>GQDMVSPPPPIADEPLTVNTGIYLIECYSLDDKAETFKVNAFLSLSWKDRRLAFDPVRSGVRVKTYEPEAIWIPEIRFVNVENARAADVVDISVSPDGTVQYLERFSARVLSPLDFRRYPFDSQTLHIYLIVRSVDTRNIVLAVDLEKVGKNDDVFLTGWDIESFTAVVKPANFALEDRLESKLDYQLRISRQYFSYIPNIILPMLFILFISWTAFWSTSYEANVTLVVSTLIAHIAFNILVETNLPKTPYMTYTGAIIFMIYLFYFVAVIEVTVQHYLKVESQPARAASITRASRIAFPVVFLLANIILAFLFFGF[5x]

At present, the best structurally characterized pLGIC is the G. violaceus ligand-gated ion channel (GLIC), of prokaryotic origin. Each subunit consists of an extracellular domain (ECD), predominantly in a β-sandwich fold, and a transmembrane domain (TMD) composed of four helices, labeled M1–M4. However, the GLIC is a pH-gated channel, activated by lowering the pH, with a maximal activation at pH 4 and a pH50 around 5. We instead found that proton activation is a complex multiple loci mechanism, with the key contribution stemming from the coupling interface between the extracellular and transmembrane domain, with E35 acting as a key proton-sensing residue.

The mutant of the vestibular pair on the β5 strand, D86N-D88N, yields a significant decrease in pH50 greater than 1 pH unit. All residues were also tested individually, with most mutations having no significant effect, although a large majority tend to decrease the pH50 (notably D86N/A, D88N/A, and D91N). Mutation of Asp/Glu residues at the complementary (−) face, in general, decreased the proton sensitivity of the GLIC, with additive effects in many cases, especially for D88 and D86. However, the pattern of phenotypes does not allow discriminating whether those residues are involved in proton sensing or gating, because mutations to Asn/Gln also produced decreased proton sensitivity. A structural analysis was performed on E26Q, E26A, E35Q, E35A, E67A, E75A, E82Q, E82A, D86A, D88N, D88A, H127N, E181A, and H277Q mutants, by solving their structure at pH 4. The key mutants at E26, D86, and D88 were solved at pH 4, each showing a structure similar to that of the Wt. All structures were in the apparently open conformation.>[2x]APDSVDYRKKGYVTPVKNQGQCGSCWAFSSVGALEGQLKKKTGKLLNLSPQNLVDCVSE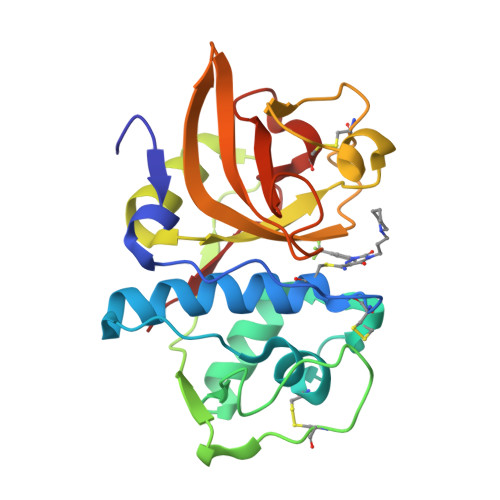NDGCGGGYMTNAFQYVQKNRGIDSEDAYPYVGQEESCMYNPTGKAAKCRGYREIPEGNEKALKRAVARVGPVSVAIDASLTSFQFYSKGVYYDESCNSDNLNHAVLAVGYGIQKGNKHWIIKNSWGENWGNKGYILMARNKNNACGIANLASFPKM> MIRDIIRMGDKRLLRVAPQVTNLGSAELHALV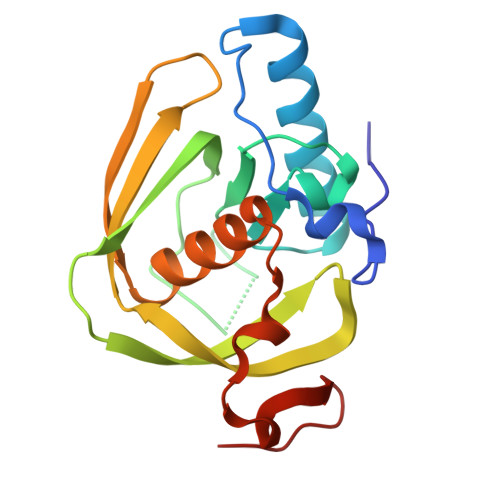SDMFETMGAAHGVGLAAPQIAVDLQLMVFGFEASERYPEAPAVPLTALANAQIEPLSDEMENGWEGCLSIPGLRAVIPRYRYIRYRGFAPDGSPIEREAEGFHARVVQHEYDHLVGRLYPSRIENFDTFGFDDVLSYDL> SLSQNLGNTENPRPSKVQELSVYEINDLDRHSPKILKNAFSFRFGLGDLVPFTNKLYTGDLKKRVGITAGLCVVIEHVPEKNGDRFEATYSFYFGDYGHLSVQGPYLTYEDSFLAITGGAGIFEGAYGQVKLQQLVYPTKLFYTFYLKGLANDLPLELIGTPVPPSKDVEPAPEAKALKPS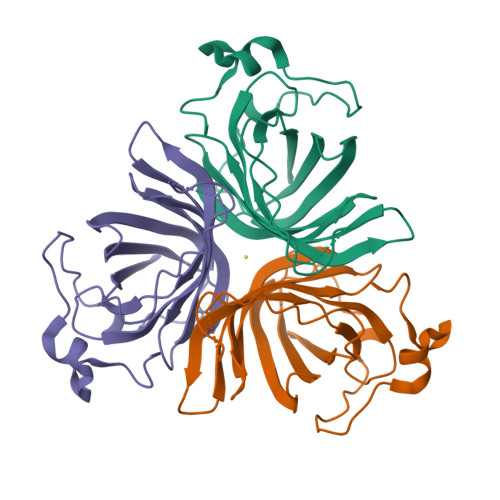GVVSNFTN> LPAYNSDIQQALKWLHNQAPGITGLIQRKAQW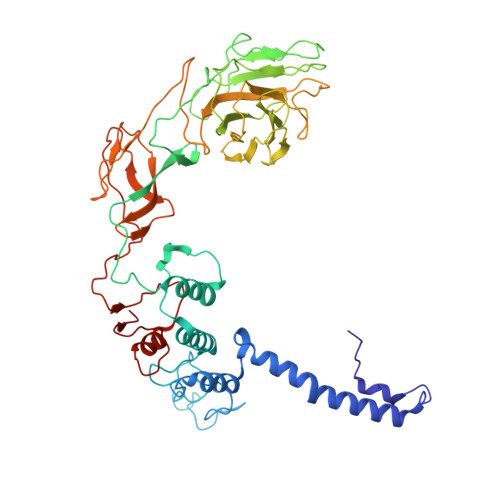YDRFSRQFWANWERDVFHLKTANPFGLMVWCIILGTPSKGFGLYPKNSSWAFGRLRQNFIYSGTQVPPPADASPGGNFYGGGNAEILNLDEIRKVLQLRYVALISNGSIAYINRMLRYIFNDDEPWDEATGLYFYLMDSTGENGPVENLAVYRKDWEGMVLLSSSPRTNHVLTSTPASDADWPGVDPAASGIPVTVETASATAPDGSATVCKLTKPAGSTAYVSAPIDGPLGSGSTVTFSFFAKAGSTRFIAIQSAADFPSRADAVFDLDSGNVISDQMLDSSVVSARMIRLENGWWRCVLTTKTVSSSFRAAYVAPAETNFSWIDSNSSAAIDVLIWGAQIELGDTPTGYLKTTGAPVTITDYVLQNAQTGTVKFTQPLPTGVEAYWTGDWKGGTAAEPARFAVGNGTQDTFTLSDPAYIGLPTSGAFKLEYRVGPALNLSPQLINLMNDRAVGIMPTCAGCDVKVI> DDNKKDDILCMASHDKGETWGTKIVIKYDNYKLGVQYFFLRPYISKNDLSFHFYVGDNINNVKNVNFIECTHEKDLEFVCSNRDFLKDNKVLQDVSTLNDEYIVSYGNDNNFAECYIFF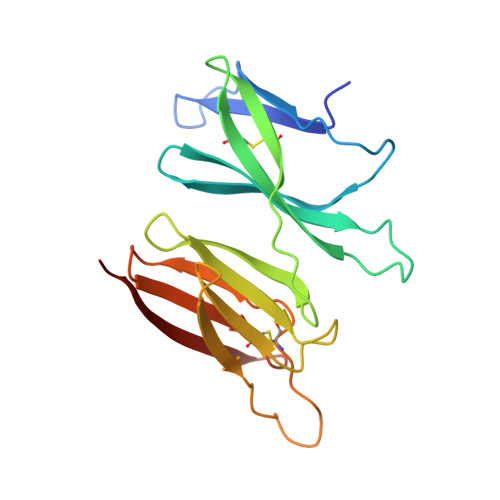NNENSILIKPEKYGQTTAGCYGGTFVKIDEQRTLFIYSSSQGIYNIHTIYYANYEEF(1R,3R,7E,17beta)-17-[(1S)-6,6,6-trifluoro-5-hydroxy-1-(4-hydroxy-4-methylpentyl)-5-(trifluoromethyl)hex-3-yn-1-yl]-9,10-secoestra-5,7-diene-1,3-diol | C31 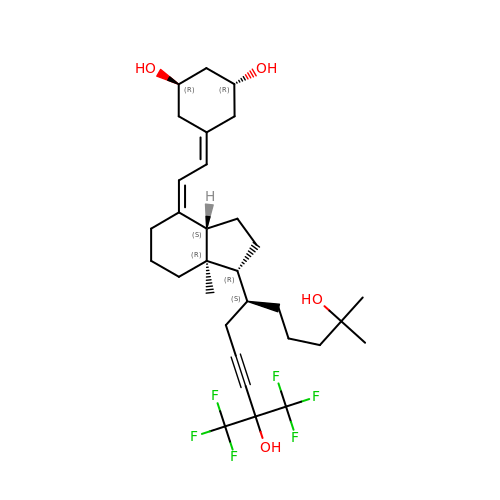H44 F6 O4 | RAYDHJNMFBHXHA-KPUKIUDSSA-N> MSAPTDDTPTDAIAAPRHSAPPRPRLPWFLRTFAVPIILAWVAVVAILNTVVPTLDEVGEMRAVSMAPNDAPSTLAIKRVGQVFEEYDTSSSVMIVLEGEEPLGIEAHAFYDKMVADLRADTEHVQHVQDFWGDTLTASGAQSVDGKAAYVQVYIAGDQGESLANESVEAVRKIATERETPSGVKAYVTGAAATSADQRAEGDASMKLIEGVTFAVITVMLLAVYRSVITTL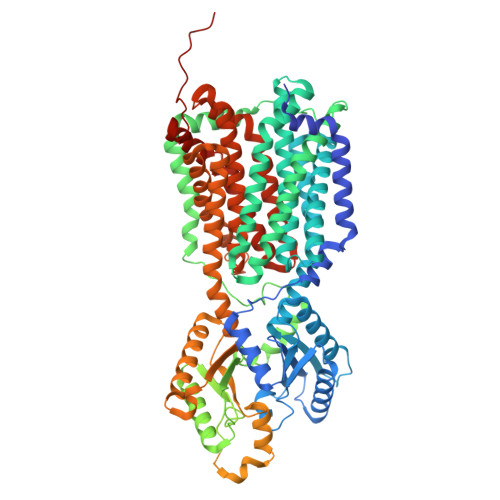IVLAMVVLGLSGARGIVAFLGFYNVFGLTTFATNMVVTLAIAAATDYAIFLIGRYQEARRAGEDRESAYYTMFHGTAHVVLASGLTIAGATLCLHFTRLPYFQTMGVPLAIGMLIVVAAALTAGPAVISVVSRFGKTLEPKRFSRSPGWHRVGTATVRWPGAILVCAVVAALIGLLALPGYYTTYDDRRYLPDDVPANVGYDAAFRHFSQAKMNPDLMMVETDRDLRNPADFLVIDKIAKALKNVHGIAQVQTITRPDGDPIEHSTIPYTIGQSGTTQIMNNDYMQTNLDNLLKQADDLQTSIDSMTEMMNIQTELAAVSQSMADKMAQTSDDTADVRDHLADFDDFFRPIRNYLYWEPHCYDIPMCWSMRSIFESIDGINTMSDDFQELVPEMRRMADLMPRMVAVMPAQIQSMKNQKQTLLNQYQVQKAQQDQNMAMQENATAMSQAFDAAKNDDSFYLPPEAFETDDFQRGMKLFMSPDGHAVRFTIIHQGDPLTEEGTARMDELKVAAADAIKGTPFEGARIYLGGSAATYNDMQIGADYDLIIVAASALILIFIIMMVLTRAVVAAAVIVGTVVLSLASAFGLSVLLWQHIVGIPLHWMVLPMSVIVLLAVGADYNLLLVSRMKEEIHAGIRTGIIRAMVGTGAVVTAAGLVFAFTMASMAVSSLITIGQVGTTIGLGLLFDTLVVRSLMTPSIATLLGRWFWWPQRVRERPVPSKWPTPIQRTPEEALS>[4x]MDWKKYGYNTRALHAGYEPPEQATGSRAVPIYQTTSYVFRDSDHAARLFALEEPGFIYTRIGNPTVSVLEERIAALEEGVGALAVASGQAAITYAILNIAGPGDEIVSGSALYGGTYNLFRHTLYKKSGIIVKFVDETDPKNIEEAITEKTKAVYLETIGNPGLTVPDFEAIAEIAHRHGVPLIVDNTVAPYIFRPFEHGADIVVYSATKFIGGHGTSIGGLIVDSGKFDWTNGKFPELVEPDPSYH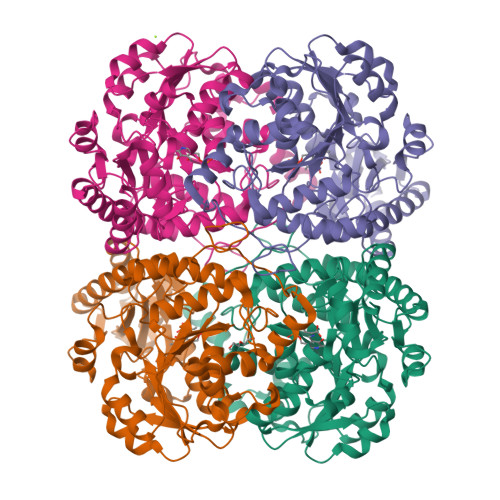GVSYVETFKEAAYIAKCRTQLLRDLGSCMSPFNAFLFILGLETLSLRMKKHCENALKIVEFLKSHPAVSWVNYPIAEGNKTRENALKYLKEGYGAIVTFGVKGGKEAGKKFIDSLTLISHLANIGDARTLAIHPASTTHQQLTEEEQLKTGVTPDMIRLSVGIEDVEDIIADLDQALRKSQEG> GSAMGSASTSGNPFQANVEMKTFMERFNLTHHHQSGIYVDLGQDKEVDGTLYREPAGLCPIWGKHIELQQPDRPPYRNNFLEDVPTEKEYKQSGNPLPGGFNLNFVTPSGQRISPFPMELLEKNSNIKASTDLGRCAEFAFKTVAMDKNNKATKYRYPFVYDSKKRLCHILYVSMQLMEGK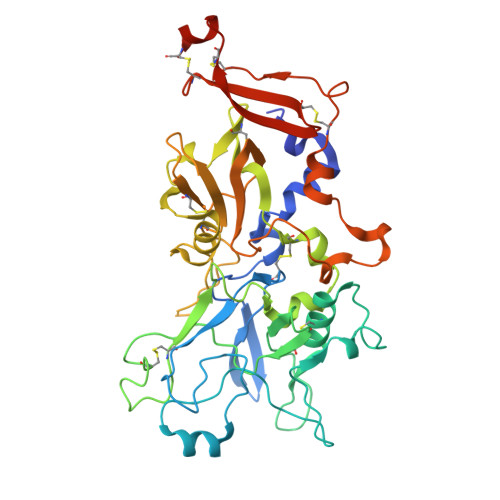KYCSVKGEPPDLTWYCFKPRKSVTENHHLIYGSAYVGENPDAFISKCPNQALRGYRFGVWKKGRCLDYTELTDTVIERVESKAQCWVKTFENDGVASDQPGSGSGSGDQPHSGGVGRNYGFYYVDTTGEGKCALSDQVPDCLVSDSAAVSYTAAGSLSEETPNFIIPSNPSVTPPTPETALQCTADKFPDSFGACDVQACKRQKTSCVGGQIQSTSVDCTADEQNECGSNTAAALVPR>MSVVSKGLENVIIKVTNLTFIDGEKGILRYRGYNIEDLVNYGSYEETIYLMLYGKLPTKKELNDLKAKLNEEYEVPQEVLDTIYLMPKEADAIGLLEVGTAALASIDKNFKWKENDKEKAISIIAKMATLVANVYRRKEGNKPRIPEPSDSFAKSFLLASFAREPTTDEINAMDKALILYTDHEVPASTTAALVAASTLSDMYSSLTAALAALKGPLHGGAAEEAFKQFIEIGDPNRVQNWFNDKVVNQKNRLMGFGHRVYKTYDPRAKIFKKLA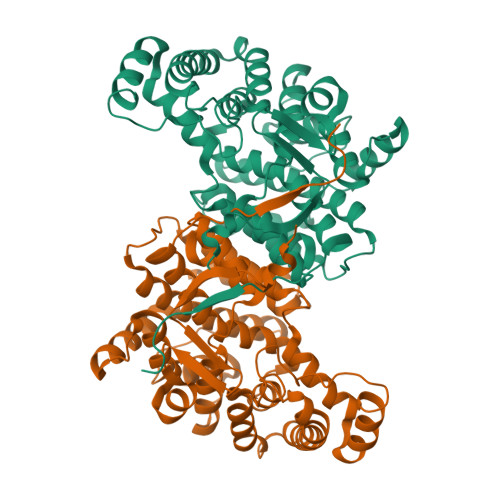LTLIERNADARRYFEIAQKLEELGIKQFSSKGIYPNTDFYSGIVFYALGFPVYMFTALFALSRTLGWLAHIIEYVEEQHRLIRPRALYVGPEYQEYVSIDKR[4x]GatD has sequence similarities to the catalytic domains of glutamine amidotransferases, while MurT is similar in sequence to the substrate-binding domains of Mur ligases. Together, these two proteins catalyze the amidation of α-D-isoglutamic acid of cell wall precursor stem peptides in an ATP-dependent reaction. In order to provide insight into the overall organization of this complex and to facilitate an understanding of the amidation mechanism, we have determined the crystal structure of the GatD/MurT complex. We find that the two proteins assemble into a curved, boomerang-shaped structure, with GatD docking to the C-terminal domain of MurT.

The native structure of the GatD/MurT complex was solved at a resolution of 2.04 Å using single isomorphous replacement with anomalous scattering (SIRAS). The refined structure has excellent statistics and includes all residues of the expressed proteins with the exception of MurT residues 1–35, 195–196 and 434–437. These regions are poorly visible in the electron density maps and therefore likely have multiple conformations and increased mobility. The GatD/MurT heterodimer adopts a boomerang-shaped conformation, with GatD packing against the C-terminal domain of MurT. Extensive interactions between GatD and MurT establish a large, continuous interface that buries a total surface area of 940 Å2 from solvent (calculated with PISA28). Instead, GatD-H189 is shifted towards the heterodimer interface, where it contacts an aspartic acid (D349) of MurT, thus establishing a possible alternative catalytic triad (GatD-C94, GatD-H189, MurT-D349) involving residues from both GatD and MurT. The close proximity of the side chains of GatD-C94 and GatD-H189 (3.7 Å) and GatD-His189 and MurT-D349 (3.1 Å) as well as their relative orientation suggest that these three residues might indeed function as a proton relay system in catalysis. The crystal structure of GatD bound to MurT establishes an initial framework for probing the function of this enzyme complex and for developing strategies to intervene with amidation. The two proteins assemble into an elongated complex, with a large open space separating GatD from the middle domain of MurT. The refined model retains the overall characteristics of the crystal structure, but it has a more compact conformation with a closest distance between GatD and the MurT middle domain, measured at the top of the structure, of 22 Å instead of 32 Å. These experiments show that, while the conformation of the unliganded GatD/MurT complex is indeed open and elongated as observed in the crystal structure, the complex can breathe somewhat in solution. The almost linear arrangement between the two MurT domains appears to be unique to MurT as all other known conformations of this two-domain segment are more closed in Mur ligases.

>MHELTIYHFMSDKLNLYSDIGNIIALRQRAKKRNIKVNVVEINETEGITFDECDIFFIGGGSDREQALATKELSKIKTPLKEAIEDGMPGLTICGGYQFLGKKYITPDGTELEGLGILDFYTESKTNRLTGDIVIESDTFGTIVGFENHGGRTYHDFGTLGHVTFGYGNNDEDKKEGIHYKNLLGTYLHGPILPKNYEITDYLLEKACERKGIPFEPKEIDNEAEIQAKQVLIDRANRQKKSRLEHHHHHH[2x];>[2x]MRQWTAIHLAKLARKASRAVGKRGTDLPGQIARKVDTDVLRKLAEQVDDIVFISGTNGKTTTSNLIGHTLKANNIQIIHNNEGANMAAGITSAFIMQSTPKTKIAVIEIDEGSIPRVLKEVTPSMMVFTNFFRDQMDRFGEIDIMVNNIAETISNKGIKLLLNADDPFVSRLKIASDTIVYYGMKAHAHEFEQSTMNESRYCPNCGRLLQYDYIHYNQIGHYHCQCGFKREQAKYEISSFDVAPFLYLNINDEKYDMKIAGDFNAYNALAAYTVLRELGLNEQTIKNGFETYTSDNGRMQYFKKERKEAMINLAKNPAGMNASLSVGEQLEGEKVYVISLNDNAADGRDTSWIYDADFEKLSKQQIEAIIVTGTRAEELQLRLKLAEVEVPIIVERDIYKATAKTMDYKGFTVAIPNYTSLAPMLEQLNRSFEGGQS N-(2-chloro-5-{[4-(trifluoromethoxy)phenyl]sulfamoyl}phenyl)-3,5-difluorobenzamide | C20 H12 Cl F5 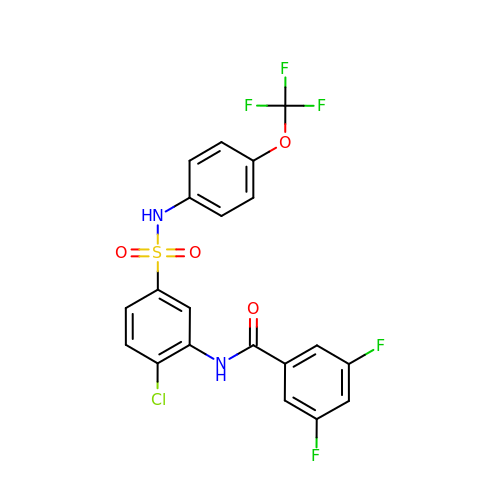N2 O4 S | HMZYFFHZWUTOLH-UHFFFAOYSA-N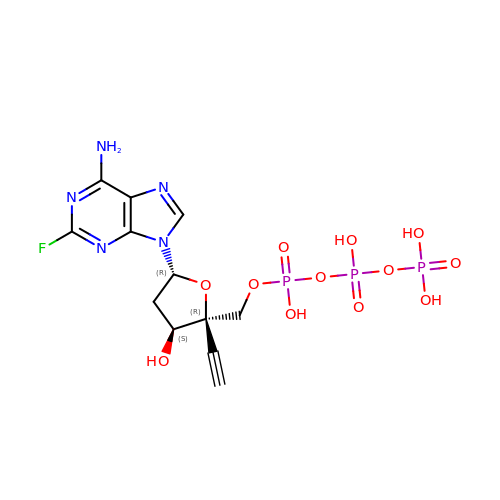2'-deoxy-4'-ethynyl-2-fluoroadenosine 5'-(tetrahydrogen triphosphate) | C12 H15 F N5 O12 P3 | BUMPFXRZUYYODO-QRPMWFLTSA-N>MRVVIQRVKGAILSVRKENIGENEKELEIISEIKNGLICFLGIHKNDTWEDALYIIRKCLNLRLWNNDNKTWDKNVKDLNYELLIVSQFTLFGNTKKGNKPDFHLAKEPNEALIFYNK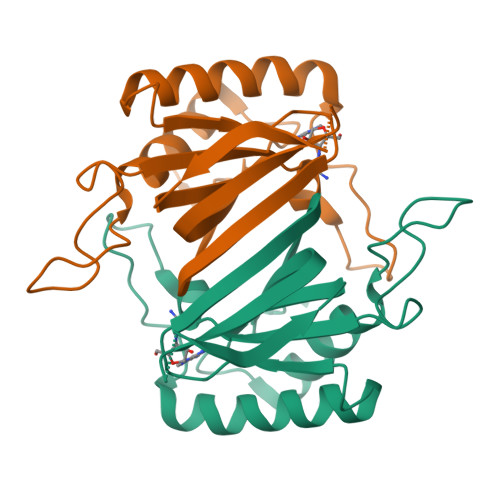IIDEFKKQYNDDKIKIGKFGNYMNIDVTNDGPVTIYIDTHDINLNK[8x]>[10x]MLLIGKPAPHFSANAVVNGTIVPDFSLDQFKGKKYVILFFYPKDFTFVCPTELIGFQEALGEFDKRDVAVVGC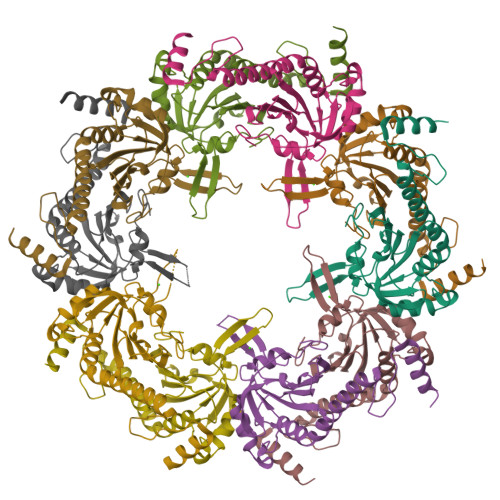STDSEFSHWAWVNTPRDQGGIQGVSYPIVSDINKTISADYGVLAGDEEIDEDGNVEVNGELIAYRGLFLIDKDGIVRHQLINDFPLGRSIDEAIRVVDALQHFELYGEVCPLGWHKGEAAMTPSHEGVASYLSKLEHHHHHH> DVSGTVCLSALPPEATDTLNLIASDGPFPYSQDGVVFQSRESVLPTQSYGYYHEYTVITPGARTRGTRRIITGEATQEDYYTGDHYAT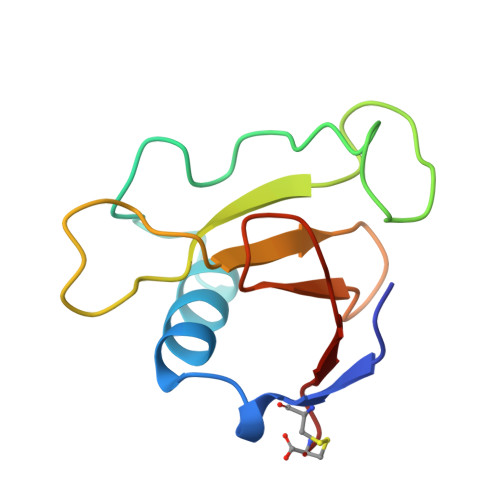FSLIDQTC>[2x]MNTVRSEKDSMGAIDVPADKLWGAQTQRSLEHFRISTEKMPTSLIHALALTKRAAAKVNEDL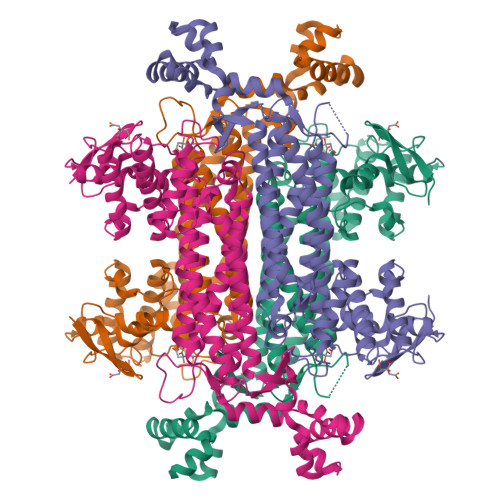GLLSEEKASAIRQAADEVLAGQHDDEFPLAIWQTGSGTQSNMNMNEVLANRASELLGGVRGMERKVHPNDDVNKSQSSNDVFPTAMHVAALLALRKQLIPQLKTLTQTLNEKSRAFADIVKIGRTHLQDATPLTLGQEISGWVAMLEHNLKHIEYSLPHVAELALGGTAVGTGLNTHPEYARRVADELAVITCAPFVTAPNKFEALATCDALVQAHGALKGLAASLMKIANDVRWLASGPRCGIGEISIPENEPGSSIMPGKVNPTQCEALTMLCCQVMGNDVAINMGGASGNFELNVFRPMVIHNFLQSVRLLADGMESFNKHCAVGIEPNRERINQLLNESLMLVTALNTHIGYDKAAEIAKKAHKEGLTLKAAALALGYLSEAEFDSWVRPEQMVGSMKAGRHHHHH> MNPFQKNESKETLFSPVSIEEVPPRPPSPPKKPSPTICGSNYPLSIAFIVVNEFCERFSYYGMKAVLILYFLYFLHWNEDTSTSIYHAFSSLCYFTPILGAAIADSWLGKFKTIIYLSLVYVLGHVIKSLGALPILGGQVVHTVLSLIGLSLIALGTGGIKPCVAAFGGDQFEEKHAEERTRYFSVFYLSINAGSLISTFITPMLRGDVQCFGEDCYALAFGVPGLLMVIALVVFAMGSKIYNKPPPEGNIVAQVFKCIWFAISNRFKNRSGDIPKRQHWLDWAAEKYPKQLIMDVKALTRVLFLYIPLPMFWALLDQQGSRWTLQAIRMNRNLGFFVLQPDQMQVLNPLLVLIFIPLFDFVIYRLVSKCGINFSSLRKMAVGMILACLAFAVAAAVEIKINEMAPAQPGPQEVFLQVLNLADDEVKVTVVGNENNSLLIESIKSFQKTPHYSKLHLKTKSQDFHFHLKYHNLSLYTEHSVQEKNWYSLVIREDGNSISSMMVKDTESRTTNGMTTVRFVNTLHKDVNISLSTDTSLNVGEDYGVSAYRTVQRGEYPAVHCRTEDKNFSLNLGLLDFGAAYLFVITNN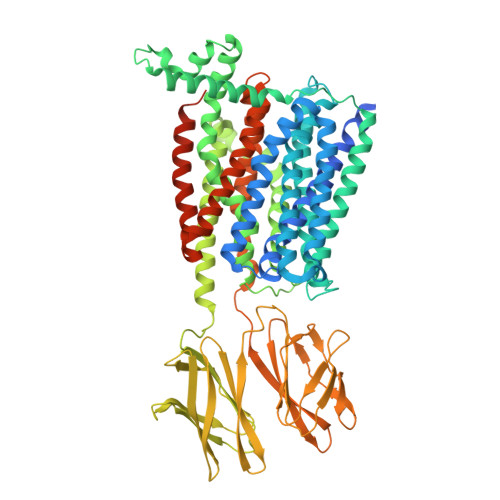TNQGLQAWKIEDIPANKMSIAWQLPQYALVTAGEVMFSVTGLEFSYSQAPSSMKSVLQAAWLLTIAVGNIIVLVVAQFSGLVQWAEFILFSCLLLVICLIFSIMGYYYVPVKTEDMRGPADKHIPHIQGNMIKLETKKTKL beta-D-galactofuranose | C6 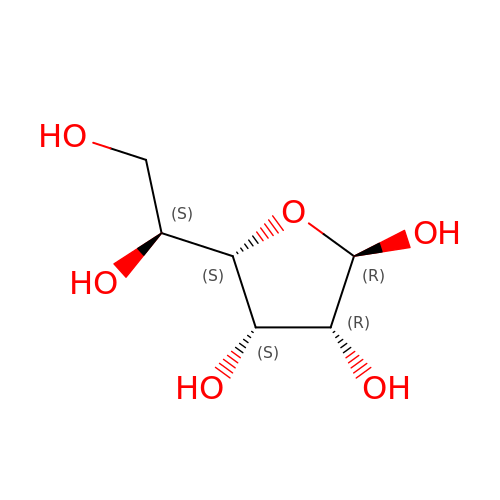H12 O6 | AVVWPBAENSWJCB-DGPNFKTASA-N> MIVDEFSSVYECLLYCYKMVKRSEQLNGRRVFPILSVVTNNNDPEGRRRVKIADPLFGNLIESNWIRPIRVSQNQDNPLPQINQMVIVWFVDGDSEKGYYLPIINDANPSREKDDPVNDSAVRIEGNNTIRIDKNDSETVGGNQTVAIAGEQNINVDGNLIENIGGDIDQ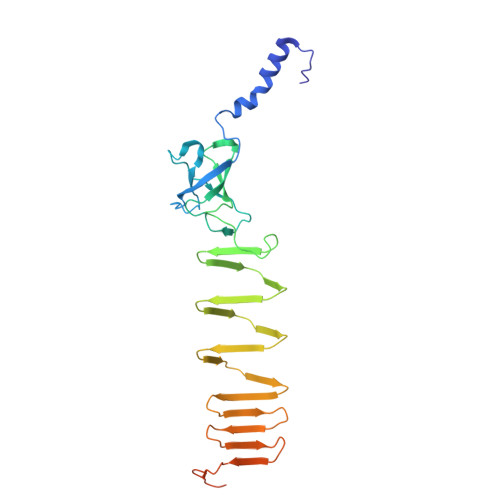NVTGKIEVRSESTILIDADGTIIIKNDSGAFISLGGNGEVLIQDSQGRKIRLGGAFNSTWDLNGLPMAFINATSVTIAGKQIATVGAVDTRGDTIVNKGW> PKEYDDELTF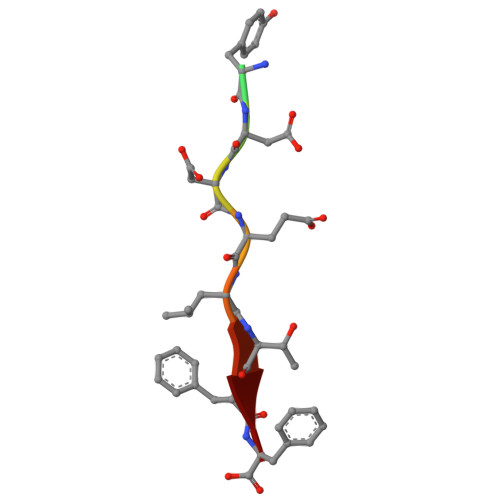F(1S,5S,6R)-10-[(3,5-dichlorophenyl)sulfonyl]-3-[2-(3,4-dimethoxyphenoxy)ethyl]-5-ethyl-3,10-diazabicyclo[4.3.1]decan-2-one | C26 H32 Cl2 N2 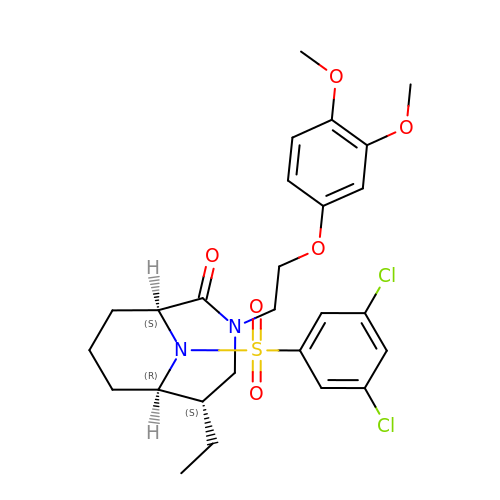O6 S | SOAFFLJOXUCIRE-IMRHEYAYSA-N>[2x]MRKALITGASRGIGRAIALRLAEDGFALAIHYGQNREKAEEVAEEARRRGSPLVAVLGANLLEAEAATALVHQAAEVLGGLDTLVNNAGITRDTLLVRMKDEDWEAVL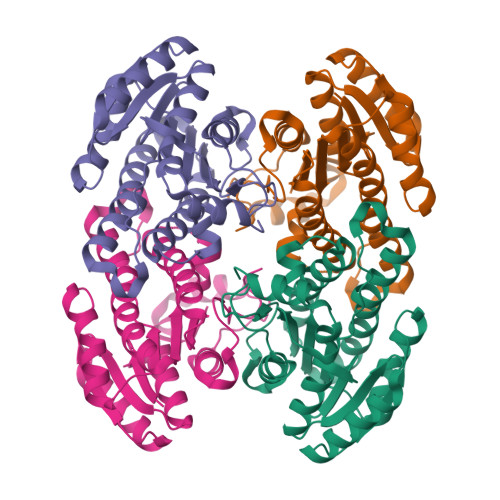EANLSAVFRTTREAVKLMMKARFGRIVNITSVVGILGNPGQANYVASKAGLIGFTRAVAKEYAQRGITVNAVAPGFIETEMTERLPQEVKEAYLKQIPAGRFGRPEEVAEAVAFLVSEKAGYITGQTLCVDGGLTPH>[4x]GSEFMTEAALVEGQVKLRDGKKWKSRWLVLRKPSPVADCLLMLVYKDKCE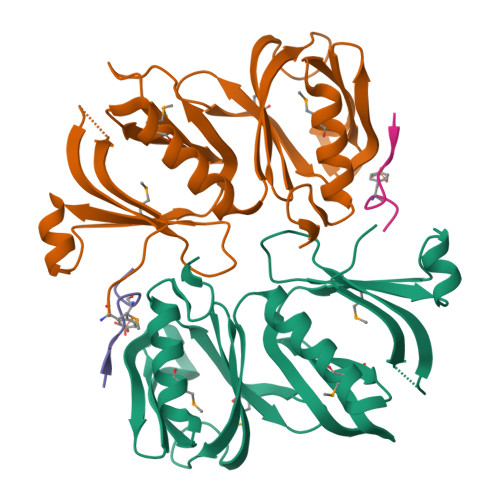RSKGLRERSSLTLEDICGLEPALPYEGLAHTLAIICLSQAVMLGFDSHEAMCAWDTRIRYALGEVHRFHVTVAPGTKLESGPATLHLCNDILVLARDIPPTVMGQWKLSDLRRYGAVPNGFIFEGGTRCGYWAGVFFLSSAEGEQMSFLFDCIVRGISPTKGPFGLRPVLPDPS;>LDRLHPNPMYQRM[4x]>GSRRASVGSHRFKVHNYMSPTFCDHCGSLLWGLVKQGL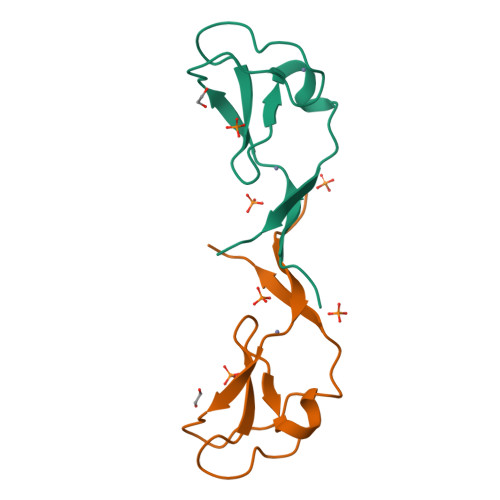KCEDCGMNVHHKCREKVANLCEFIVTD[2x]> GEQLQAWRWEREIDERNRPLSDEE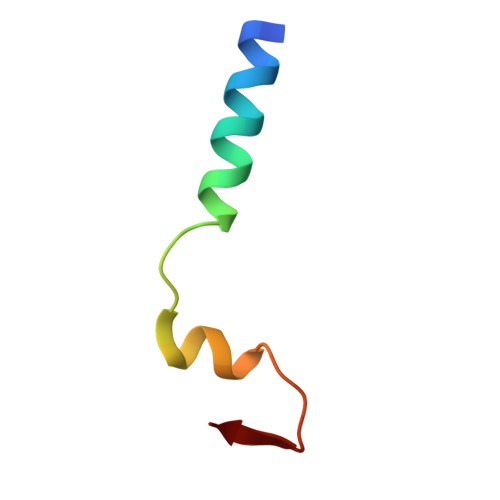LDAMFPEGYKVL>[2x]DDLYRQSLEIISRYLREQATGSKDTKPL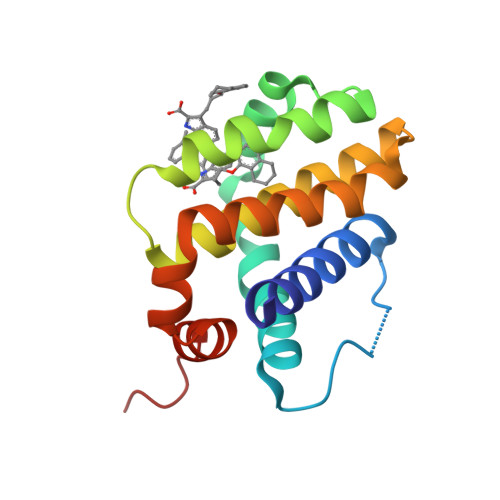GEAGAAGRRALETLRRVGDGVQRNHETAFQGMLRKLDIKNEDDVKSLSRVMIHVFSDGVTNWGRIVTLISFGAFVAKHLKTINQESCIEPLAESITDVLVRTKRDWLVKQRGWDGFVEFFHVEDLE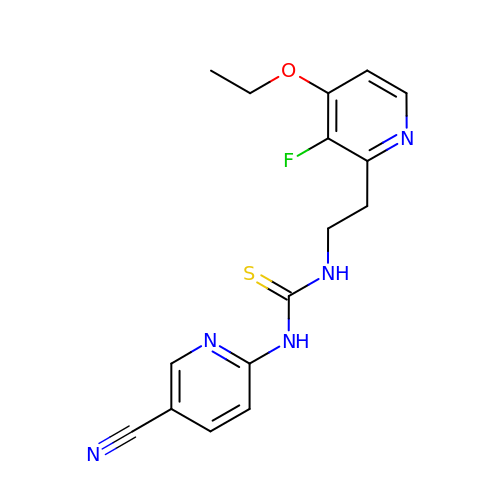N-[[3-FLUORO-4-ETHOXY-PYRID-2-YL]ETHYL]-N'-[5-NITRILOMETHYL-PYRIDYL]-THIOUREA | C16 H16 F N5 O S | PQSCCWFMTRVFDA-UHFFFAOYSA-N> GPGSHLAHPNLDTFTPEELLQQMKELLTK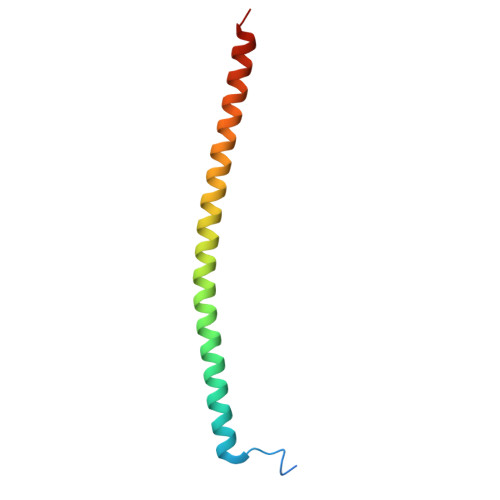NHQLKEAMKLNNQAMKGRFEELSAWTEKQKEERQFFEIQSKEAKERLMALSHE>[8x]MAHHHHHHMIVEERIYDLRPNGAREFAQHFEREGIAIQRPVL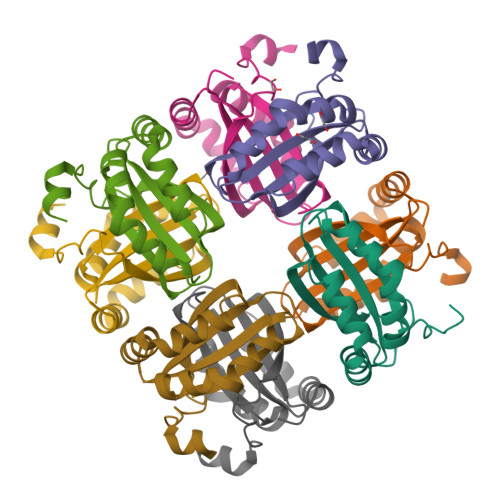GRLIGYFYTDIGPLNQVVHLWGYEDLEDRARRRAILLAMPEWQEYVRKNIQPLLVRMQNKILLPMSFSPPLPPLWQPEDEHARR> SELRPSGDSGSSDVDAEISDGFSPLDTSHRDVADEGSLLRRAEMYQDYMKQVPIPTNRGSLIPFTSWVGLSISMKQ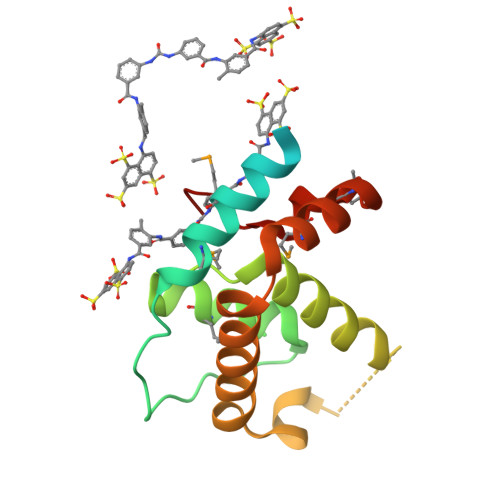LYGQPLHYLTNVLLQRWDQSRFGTDSEEQRLDSIIHPTKAEATIWLVEEIHRLTPSHLHMALLWRSDPMYHSFIDPIFPEK(3R,4R)-1-SULFAMOYL-PYRROLIDINE-3,4-DICARBOXYLIC ACID 3-[(4-CHLORO-PHENYL)-AMIDE] 4-{[2-FLUORO-4-(2-OXO-2H-PYRIDIN-1-YL)-PHENYL]-AMIDE} | C23 H21 Cl F N5 O5 S | 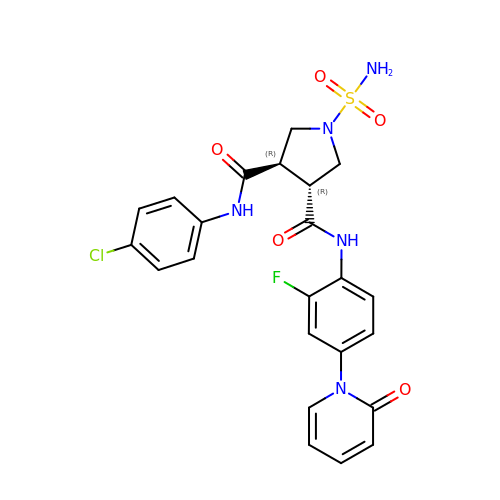GYWPDZGVFZEVMA-ROUUACIJSA-N>MRVPEKYSTLPAEDRSVHIVNICAIEDLGYLPSEGTLLNSLSVDPDAECKYGLYFRDGKRKVDYILVYHHKRASGSRTLARRGLQNDMVLGTRSVRQDQPLPGKGSPVDAGSPEVPMDYHEDDKRFRREEYEGNLLEAGLELENDEDTKIHGVGFVKIHAPWHVLCREAEFLKLKMPTKKVYHISETRGLLKTINSVLQKITDPIQPKVAEHRPQTTKRLSYPFSREKQHLFDLTDRDSFFDSKTRSTIVYEILKRTTCTKAKYSMGITSLLANGVYSAAYPLHDGDYEGDNVEFNDRKLLYEEWASYGVFYKYQPIDLVRKYFGEKVGLYFAWLGAYTQMLIPASIVGVIVFLYGCATVDENIPSMEMCDQRYNITMCPLCDKTCSYWKMSSACATARASHLFDNPATVFFSVFMALWAATFMEHWKRKQMRLNYRWDLTGFEEEEEAVKDHPRAEYEARVLEKSLRKESRNKETDKVKLTWRDRFPAYFTNLVSIIFMIAVTFAIVLGVIIYRISTAAALAMNSSPSVRSNIRVTVTATAVIINLVVIALLDEVYGCIARWLTKIEVPKTEKSFEERLTFKAFLLKFVNSYTPIFYVAFFKGRFVGRPGDYVYIFRSFRMEECAPGGCLMELCIQLSIIMLGKQLIQNNLFEIGIPKMKKFIRYLKLRRQSPSDREEYVKRKQRYEVDFNLEPFAGLTPEYMEMIIQFGFVTLFVASFPLAPLFALLNNIIEIRLDAKKFVTELRRPVAIRAKDIGIWYNILRGVGKLAVIINAFVISFTSDFIP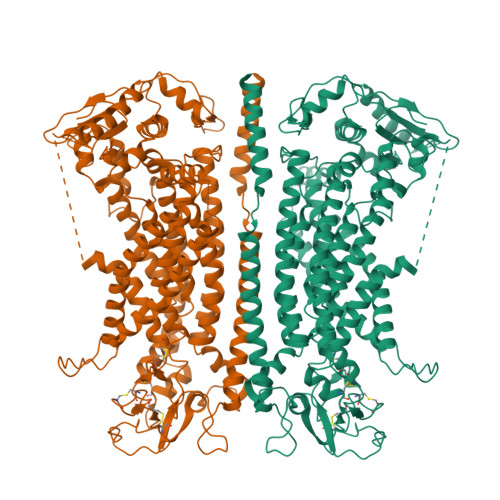RLVYLYMYSQNGTMHGFVNHTLSSFNVSDFQNGTAPNDPLDLGYEVQICRYKDYREPPWSEHKYDISKDFWAVLAARLAFVIVFQNLVMFMSDFVDWVIPDIPKDISQQIHKEKVLMVELFMREEQGKQQLLDTWMEKEKPRDVPCNNHSPTTHPEAGDGSPVPSYEYHGDAL[2x]(2S)-2-cyclohexyl-2-[2-(2,6-dimethoxypyridin-3-yl)-5,6-difluoro-1H-benzimidazol-1-yl]-N-(trans-4-hydroxycyclohexyl)acetamide 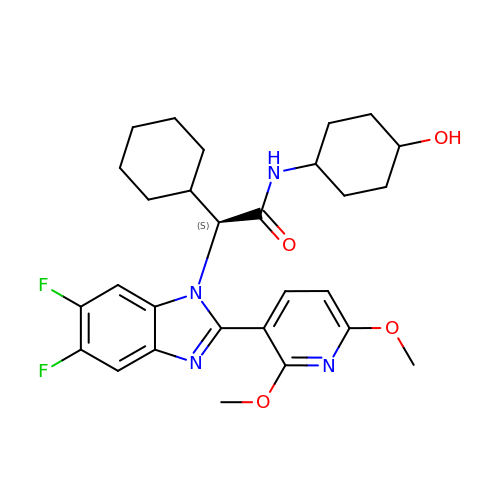| C28 H34 F2 N4 O4 | JBIUFHDYJMTSIW-RPPIVITFSA-N> GSHMWSQNDAMAFGSQALATAFNLDFVHYRSQISSLSPRFSDEGFAGYVNALQASNILETIKKEKMNLTATTGAGVLVRQGQMSDGVWFWTFQYPVRMRLVGQTTSKPEQSFVFEITIQRVDPRLKPSGMEIRQMISRNAGPNS

DotI is a 23 kDa inner membrane protein essential for intracellular growth of L. pneumophila within mammalian and protozoan cells. DotI has one transmembrane domain in its N-terminal region, followed by a periplasmic domain13. DotI is conserved in all of the identified type IVB secretion systems, including the conjugation systems of R64 and related plasmids. Structural analysis of the periplasmic domains of DotI and its R64 ortholog TraM demonstrated that DotI and TraM are structural homologs of the T4ASS protein VirB8.

To gain insight into the role(s) of DotI in type IVB secretion, we determined the crystal structures of the C-terminal periplasmic domains of DotI (residues 73-212, DotIC) and its conjugative plasmid R64 ortholog TraM (residues 91-230, TraMC). The structure of TraMC was determined at 1.5 Å resolution with the working R and the free R factor of 18.0% and 20.7%, respectively. The crystallographic asymmetric unit contains a single molecule. As expected from the considerable amino-acid sequence similarity between DotIC and TraMC (30% identity, 54% similarity), the structure of TraMC is similar to that of DotIC. They can be superimposed with an rmsd (root mean square deviation) for corresponding Cα atoms (106 of 137 atoms) of 0.876 Å. The remarkable structural difference is the position of α3. α3 of TraMC leans to Sh2, thereby closing the cleft. The conjugal plasmid R64 has no counter part of DotJ, thus TraM is expected to assemble into a homomultimer. To elucidate the oligomerization of TraM, we expressed and purified TraM using an E. coli expression system, and conducted SEC-MALS measurement. Considering the molecular weight of TraM (26 kDa) and DDM (0.5 kDa), TraM in solution is in a hexameric state with about 90 detergent molecules. The exact oligomeric state of the DotI-DotJ complex remains to be clarified, whereas TraM clearly forms a hexameric homo-oligomer.> MTGITNVTVLGTGVLGSQIAFQTAFHGFAVTAYDINTDALDAAKKRFEGLAAVYEKE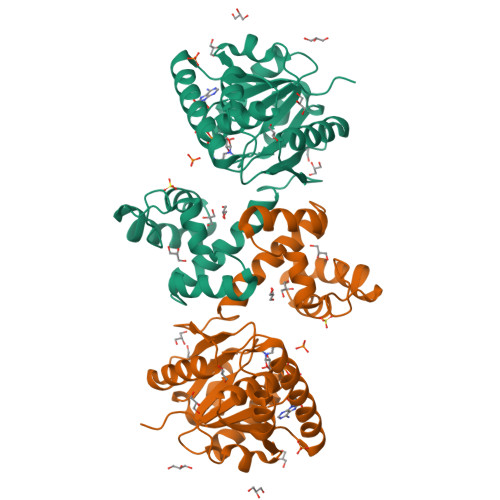VAGAADGAAQKALGGIRYSDDLAQAVKDADLVIEAVPESLDLKRDIYTKLGELAPAKTIFATNSSTLLPSDLVGYTGRGDKFLALHFANHVWVNNTAEVMGTTKTDPEVYQQVVEFASAIGMVPIELKKEKAGYVLNSLLVPLLDAAAELLVDGIADPETIDKTWRIGTGAPKGPFEIFDIVGLTTAYNISSVSGPKQREFAAYLKENYIDKGKLGLATGEGFYRY> MVYQVKDKADLD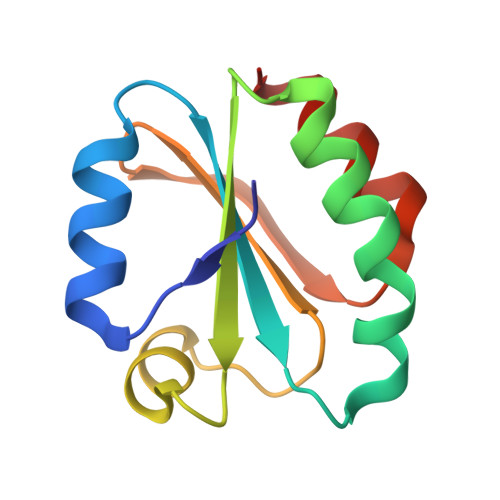GQLTKASGKLVVLDFFATWCGPCKMISPKLVELSTQFADNVVVLKVDVDECEDIAMEYNISSMPTFVFLKNGVKVEEFAGANAKRLEDVIKANI>PAMSNVPHKSSLPEGIRPGTVLRIRGLVPPNASRFHVNLLCGEEQG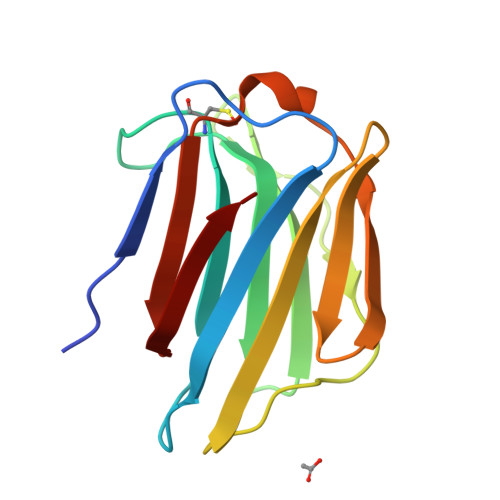SDAALHFNPRLDTSEVVFNSKEQGSWGREERGPGVPFQRGQPFEVLIIASDDGFKAVVGDAQYHHFRHRLPLARVRLVEVGGDVQLDSVRIF[2x]> GLIVDTRDVEERVHVMRKTKLAPTVAHGVFNPEFGPAALSNKDPRLNEGVVLDEVIFSKHKGDTKMSAEDKALFRRCAADYASRLHSVLGTANAPLSIYEAIKGVDGLDAMEPDTAPGLPWALQGKRRGALIDFENGTVGPEVEAALKLMEKREYKFACQTFLKDEIRPMEKVRAGKTRIVDVLPVEHILYTRMMIGRFCAQMHSNNGPQIGSAVGCNPDVDWQRFGTHFAQYRNVWDVDYSAFDANHCSDAMNIMFEEVFRTEFGFHPNAEWILKTLVNTEHAYENKRITVEGGMPSGCSATSIINTILNNIYVLYALRRHYEGVELDTYTMISYGDDIVVASDYDLDFEALKPHFKSLGQTITPADKSDKGFVLGHSITDVTFLKRHFHMDYGTGFYKPVMASKTLEAILSFARRGTIQEKLISVAGLAVHSGPDEYRRLFEPFQGLFEIPSYRSLYLRWVNAV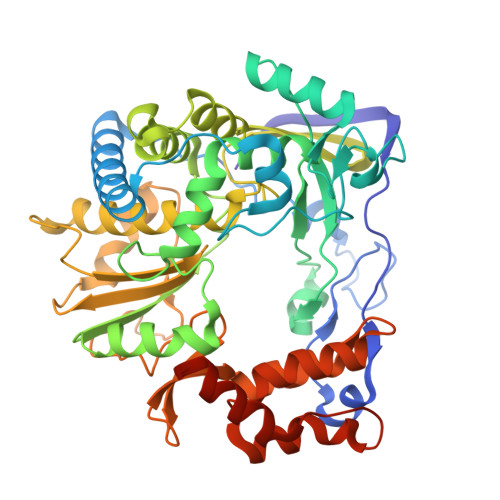CGDAAALEHHHHHH Retention of α-Tol in animals requires α-tocopherol transfer protein (α-TTP) in the liver, a cytosolic transporter of 32 kDa weight. α-TTP belongs to the Sec-14 like family, a protein group involved in secretion and lipid transfer. α-TTP recognises and selectively extracts α-Tol from the endosomal fraction of the hepatocytes allowing for its transfer into the inner leaflet of the plasma membrane and eventually across the plasma membrane into the blood-stream. Here we show that, upon binding to α-Tol, α-TTP is formed acquiring tendency to aggregation into high molecular weight oligomers. X-ray diffraction reveals a spheroidal nanoparticle formed by 24 α-TTP protomers of ≈17 nm diameter. We verify that such particles are efficiently and selectively transported through a model endothelium tissue from human umbilical vein, with a 28-fold increased flux with respect to paracellular flux.

α-TTPS crystallised exclusively when starting from monodisperse solutions of monomeric α-TTP. α-TTPS can exist in different oxidation states; we obtained crystals in both the fully reduced and the fully oxidised states. X-ray diffraction patterns indicated that both crystals belong to the space group I432, with essentially identical unit-cell parameters a = 168.18 Å (reduced) and a = 168.26 Å (oxidised). The crystal structures were solved by molecular replacement method using the atomic model of monomeric α-TTP (PDB code 1OIP39) and refined at 2.40 Å resolution (reduced form; Rwork:Rfree 18.2%:21.5%) and at 2.42 Å resolution (oxidized form; Rwork:Rfree 19.1%:21.2%) respectively. In both cases, the asymmetric unit consists of a single α-TTP molecule (residues 48–278) with one α-Tol ligand bound to it. α-TTPS is formed by 24 protomers, for a molecular mass of 0.76 MDa, assembled into a spheroidal shell reminiscent of a viral capsid. Inspection of the density map of the α-TTPS model revealed well defined density for α-Tol indicating that the protomers in the particle are bound to the ligand. The X-ray structural model of α-TTPS, for both redox states, has an external diameter of 16.8 nm consistent in size with measurements on α-TTPS particles from soluble preparations. The structure is further characterised by an apparently hollow cavity of 8.1 nm diameter. The trimeric interface is characterised by hydrophobic packing and further stabilised by salt bridges. At the very centre, the three W67 residues interact with each other in T-shape by van der Waals stacking.

> TDSFLLRFLRARDFDLDLAWRLLKNYYKWRAECPEISADLHPRSIIGLLKAGYHGVLRSRDPTGSKVLIYRIAHWDPKVFTAYDVFRVSLITSELIVQEVETQRNGIKAIFDLEGWQFSHAFQITPSVAKKIAAVLTDSFPLKVRGIHLINEPVIFHAVFSMIKPFLTEKIKERIHMHGNNYKQSLLQHFPDILPLEYGGEEFSMEDICQEWTNFIMKSEDYLSSISE>MAPTLQGQWIKVGQKGGTGPGPRSSHGIAAVGDKLYSFGGELTPNKHIDKDLYVFDFNTQTWSIAQPKGDAPTVSCLGVRMVAVGTKIYIFGGRDENRNFENFRSYDTVTSEWTFLTKLDEVGGPEARTFHSMASDENHVYVFGGVSKGGTMNTPTRFRTIEAYNIADGKWAQLPDPGDNFEKRGGAGFAVVQGKIWVVYGFATSIVPGGKDDYESNAVQFYDPASKKWTEVETTGAKPSARSVFAHAVVGKYIIIFAGEVWPDLNGHYGPGTLSNEGYALDTETLVWEKLG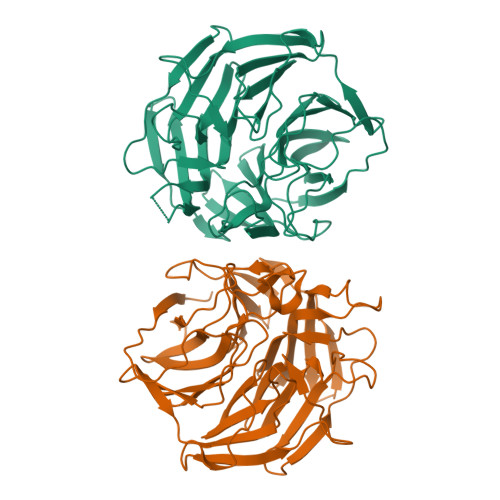EEGAPAIPRGWTAYTAATVDGKNGLLMHGGKLPTNERTDDLYFYAVNSALEHHHHHH[2x]galangin | C15 H10 O5 | 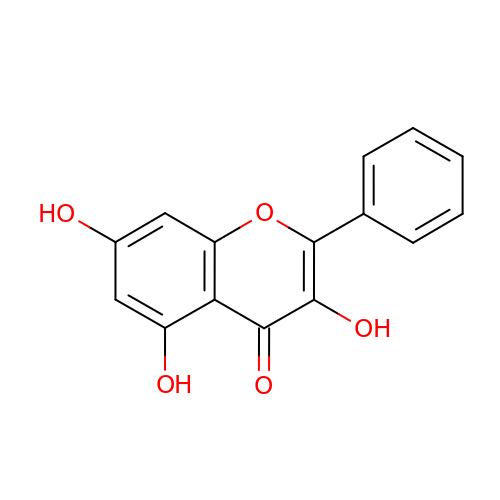VCCRNZQBSJXYJD-UHFFFAOYSA-N> GPVEDAITAAIGRVADTVGTGPTNSEAIPALTAAETGHTSQVVPGDTMQTRHVKNYHSRSESTIENFLCRSACVYFTEYENSGAKRYAEWVITPRQAAQLRRKLEFFTYVRFDLELTFVITSTQQPS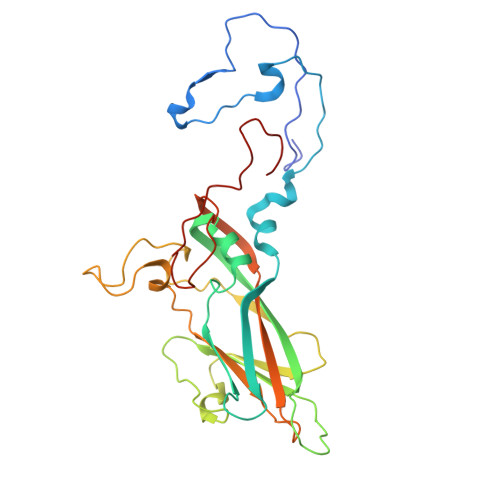TTQNQDAQILTHQIMYVPPGGPVPDKVDSYVWQTSTNPSVFWTEGNAPPRMSIPFLSIGNAYSNFYDGWSEFSRNGVYGINTLNNMGTLYARHVNAGSTGPIKSTIRIYFKPKHVKAWIPRPPRLCQYEKAKNVNFQPSGVTTTRQSITTMTNT> MGQALGIKSCDFQAARNNEEHHTKALSSRRLFVRRGQPFTIILYFRAPVRAFLPALKKVALTAQTGEQPSKINRTQATFPISSLGDRKWWSAVVEERDAQSW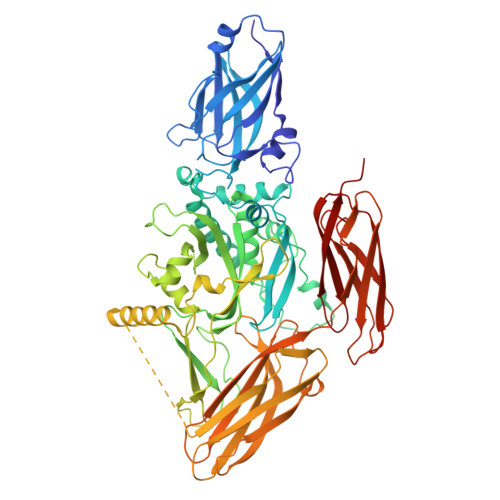TISVTTPADAVIGHYSLLLQVSGRKQLLLGQFTLLFNPWNREDAVFLKNEAQRMEYLLNQNGLIYLGTADCIQAESWDFGQFEGDVIDLSLRLLSKDKQVEKWSQPVHVARVLGALLHFLKEQRVLPTPQTQATQEGALLNKRRGSVPILRQWLTGRGRPVYDGQAWVLAAVACTVLRCLGIPARVVTTFASAQGTGGRLLIDEYYNEEGLQNGEGQRGRIWIFQTSTECWMTRPALPQGYDGWQILHPSAPNGGGVLGSCDLVPVRAVKEGTLGLTPAVSDLFAAINASCVVWKCCEDGTLELTDSNTKYVGNNISTKGVGSDRCEDITQNYKYPEGSLQEKEVLERVEKEKMEREKDNGIRPPSLETASPLYLLLKAPSSLPLRGDAQISVTLVNHSEQEKAVQLAIGVQAVHYNGVLAAKLWRKKLHLTLSANLEKIITIGLFFSNFERNPPENTFLRLTAMATHSESNLSCFAQEDIAICRPHLAIKMPEKAEQYQPLTASVSLQNSLDAPMEDCVISILGRGLIHRERSYRFRSVWPENTMCAKFQFTPTHVGLQRLTVEVDCNMFQNLTNYKSVTVVAPELSA>MASGSPPSQPSPASGSGYVPGSVSAAFVTCPNEKVAKEI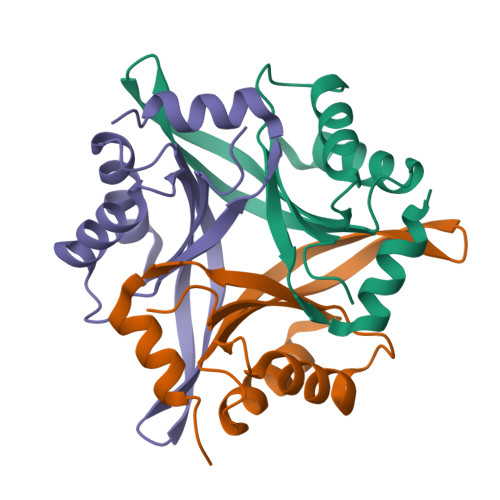ARAVVEKRLAACVNLIPQITSIYEWKGKIEEDSEVLMMIKTQSSLVPALTEFVRSVHPYEVAEVIALPVEQGNPPYLHWVHQVTESV[6x]D-Aspartate Tenofovir 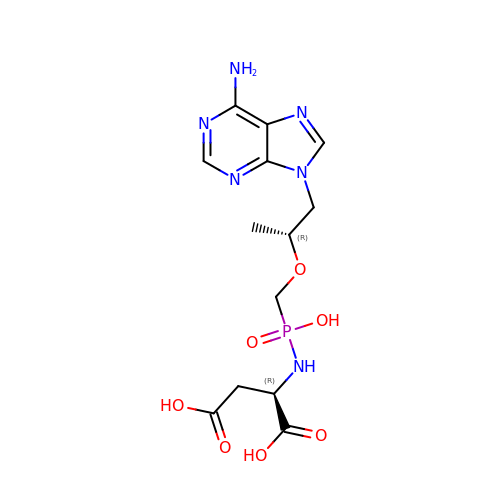| C13 H19 N6 O7 P | YBOHKRVDTZQCCV-HTQZYQBOSA-N>MRGSHHHHHHGLVPRGSMIRTMLQGKLARVKVTHADLHYEGSCAIDQDFLDAAGIL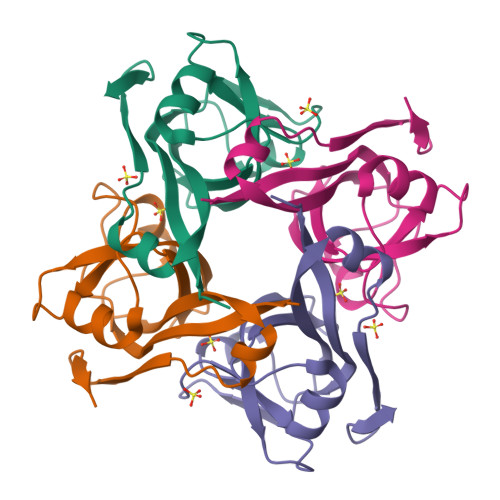ENEAIDIWNVTNGKRFSTYAIAAERGSRIISVNGAAAHCASVGDIVIIASFVTMPDEEARTWRPNVAYFEGDNEMKRTAKAIPVQVA[2x]> MYTKNFSNSRMEVKGNNGCSAPIIRKPFKHIVLTVPSSDLDNFNTVFYVQPQYINQALHLANAFQGAIDPLNLNFNFEKALQIANGIPNSAIVKTLNQSVIQQTVEISVMVEQLKKIIQEVLGLVINSTSFWNSVEATIKGTFTNLDTQIDEAWIFWHSLSAHNTSYYYNILFSIQNEDTGAVMAVLPLAFEVSVDVE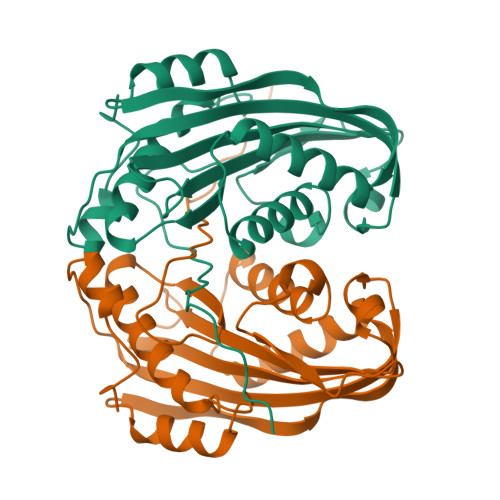KQKVLFFTIKDSARYEVKMKALTLVQALHSSNAPIVDIFNVNNYNLYHSNHKIIQNLNLSN> MSTPARRRLMRDFKRMKEDAPPGVSASPLPDNVMVWNAMIIGLADTPYEDGTFRLLLEFDEEYPNKPPHVKFLSEMFHPNVYANGEICLDILQNRWTPTYDVASILTSIQSLFNDPNPASPANVEAATLFKDHKSQYVK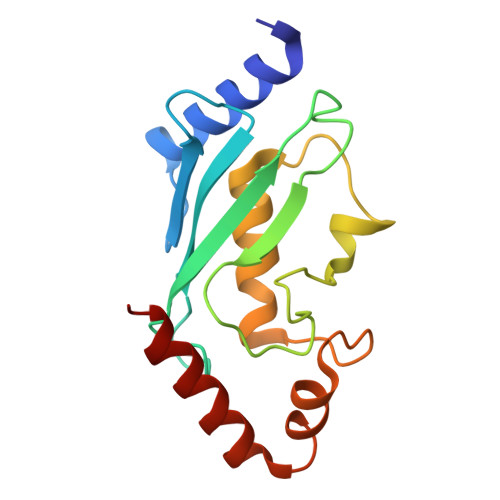RVKETVEKSWE> SMHSDLTFCEIILMEMESHDAAWPFLEPVNPRLVSGYRRIIKNPMDFSTMRERLLRGGYTSSEEFAADA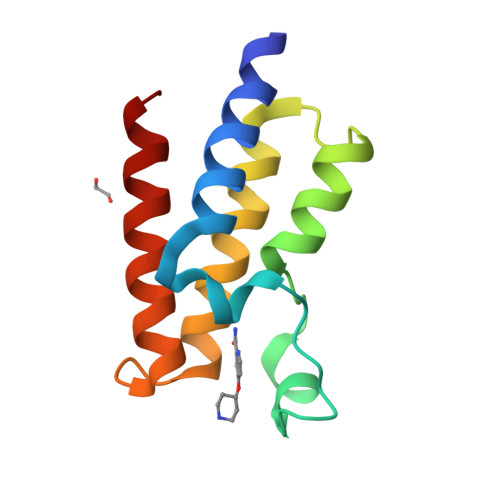LLVFDNCQTFNEDDSEVGKAGHIMRRFFESRWEEFY>[2x]MAHHHHHHMYAIGLTGGIGSGKTTVADLFAARGASLVDTDLIAHRITAPAGLAMPAIEQTFGPAFVAADGSLDRARMRALIFSDEDARRRLEAITHPLIRAETE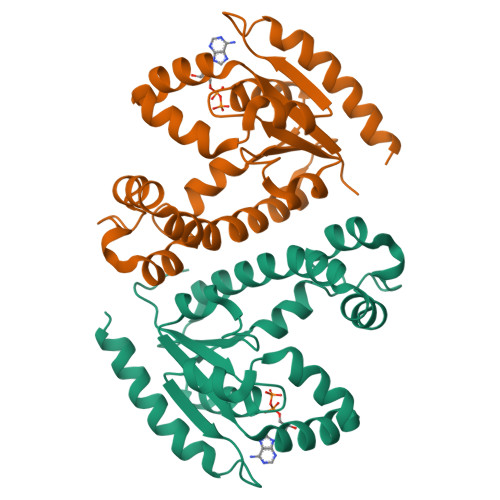REARDAQGPYVIFVVPLLVESRNWKARCDRVLVVDCPVDTQIARVMQRNGFTREQVEAIIARQATREARLAAADDVIVNDAATPDALAVQVDALHQRYLAFAAAKH> RSVVGVVNQPIDVTVTLKLGGYEPLFTMSAQQPSIVPFTPQAY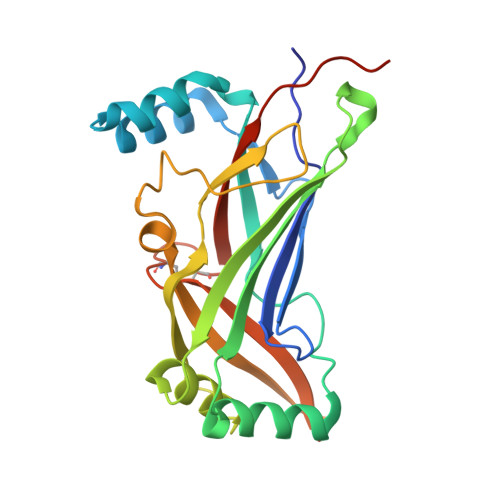EELSQQFDPYPLAMQFISQYSPEDIVTAQIEGSSGALWRISPPSRAQMKQELYNGTADITLRFTWNFQRDLAKGGTVEYTNEKHTLELAPNSTARRQLAQLLEGRPDQSVVIPHLFPKYIRAPNGPEANPVKQLQPDEEEDYLGVRIQLRREQVGTGASGEQAGTKASDFLEWWVIELQDCKADCNLLPMVIFSDKVSPPSVEHHHHHH> MNIVP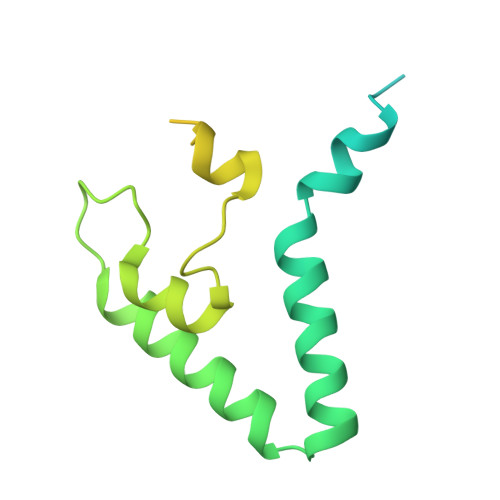QDTFKSQVSTDQDKSVLSSAVPSLPDTLRQQEGGAVPLSTQLNDRHPLESTLKNWETTQRQRQMEQYRQIFGIAEPMKRTMEMEIVNRTDFNPLSTNGSIHRDILLNKECSIDWEDVYPGTGLQASTMVGDDVHSKIEKQLGIGRRIPGLINPWKRRWKKNFIAVSAANRFKKISSSGALDYDIPTTASENLYFQ>MSQCCCLSPQEERLQGTKKVNRQGRERVYKILDRIQFTVPHVDIERARYFTESMRQTEGELLTLRWAKALKNVAEKMTVYITPDQLLAGRVGQLGRYGILYPEIDGDFYIEVMKDLPNREKSPFQIDPAAAAILMEEIAPYWEGKTYHEHLNKVLPAEIRGVTYHDERGLKSKFVVSETSSYRSALQWVPDYEKAMKRGFIDIQNEAKAKLAGLDLTNSVDIWEKKPFLEAMIIVCDAIMIWAKRHAQLARDTAAATSDPVRKQELLRMADICEHVPAYPARNFREAVQCQWFVQMFSRIEQKASAIISNGRMDQYLYPYYKKDIEEGTLTSEEAKELLECMWVDMAQFIDLYINPTGNEFQEGYAHWEAVTVGGQTPEGEDATNELSYLFLESKREFPMTYPDLAVRIHSRTPDRFLYEIALTVQDGSGFPKLINDEEVVPLNAIKGCPINEALDYAISGCTETRMPNRDTYTSGCVYINFATALEMLMNNGRLHYYGDELIGLETGDPTRFQTWEEFYEAYKAQHINLLQKAFQQQHIVDRLRPQHFAAPLSSVLHNLCMKNMQDLHSEKIEGGVDYSYFEFLGYATVVDSLAAIKKLVFEEKRLTMREVLDAMNANFVGYEPIQEMLKNAPCYGNNDPYADSIAKDVDRFTQVEAEKSSRDRGIHVDVRYVPITSHVPFGKIIAATPNGRVAGFPLADGSSASHGADHNGPTAVLLSNYHSKNYGMINRASRLLNIKLSPKCVAGEQGAKKIMSIIRTW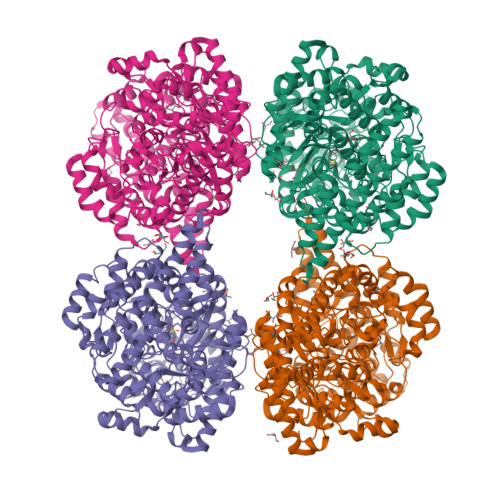CDLKLWHLQFNIVNRDTLLAAQKDPNSYRNLIVRVAGYSAYFCDMSPDLQNDIIDRTEHADL[4x]>[2x]GPAMGQTADDHNPKYEDVDVKPGETNKVTPTNTDKDGNPANIPDGTKFEKDPDAPSWVEVDPNTGELTVAPPEGTPSGGHEIKVKVTYPDGSTDEVPVTVKVSDPTTP

Proteins attached to the surface of group A and group B streptococcal human pathogens that contain tandemly arrayed Rib domains have been associated with invasive infections and proposed as potential vaccine candidates. Here, we study Rib domains from Rib, R28, and from a surface protein from Lactobacillus acidophilus. Together, these 5 structures of homologous Rib domains, and further sequence analyses, show Rib is an example of domain atrophy, a rare event in domain structural evolution involving the loss of core secondary structure elements, and also reveal the remarkable structural malleability of this domain family. The structure, molecular dynamics simulations, and small angle X-ray scattering of a Rib domain pair suggest tandemly arrayed domains are likely to form an elongated rod on the bacterial cell surface, thus suggesting a possible mechanism of immune evasion mediated through domain number variation.

We hypothesized that some members of the Rib domain that have long insertions in the position of the characteristic Rib D-E strand atrophy may retain the full Ig fold and thus represent something akin to the ancestral form of the atrophied Rib domain. Thus, we solved the structure of “Rib Long” (RibL) (residues 1165 to 1268) and “Rib Standard” (RibS) (residues 1269 to 1329) at resolutions of 1.07 Å and 1.25 Å, respectively. As predicted, the Ig-fold D/E strands missing from RibR and R28N are also missing from RibS but are present in the RibL structure. Thus, RibL comprises a full Ig-like fold which likely represents the ancestral state of the Rib domain, and RibS is an example of evolutionarily recent domain atrophy from RibL; this is remarkable because there are very few cases where we have the structure of both atrophied and nonatrophied domains that are closely related in sequence. RibS belongs to the “Rib” subfamily, giving a Cα rmsd value of 0.6 Å for superposition with both RibR and RibR28N, versus a Cα rmsd of 2.3 Å for RibL. A longer Rib domain contains the full Ig fold and likely represents an ancestral preatrophy structure, thus providing a rare example of a closely related pair of structures of an atrophied domain with its ancestral form. In the atrophy of the Ig-like RibL, a significant loss of the structure (∼20% compared to RibR/RibS) is involved, but the domains remain thermostable with melting temperatures (Tms) of 78 °C and 88 °C for RibL and RibS, respectively, and 71 °C for RibR. As Rib (RibR, R28N, and RibS), RibL, and aRib form 3 distinct Rib subfamilies, this begins to shed light on the evolutionary pathway of a fold where an ancestral Ig-like fold (RibL) has lost core secondary structures (RibR) and diversified in structure (aRib).>[2x]SMPKPIYSYSILIFMALKN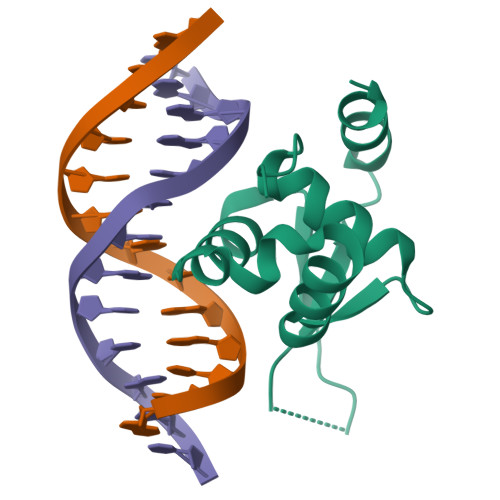SKTGSLPVSEIYNFMTEHFPYFKTAPDGWKNSVRHNLSLNKCFEKVENKSGSSSRKGCLWALNPAKIDKMQEELQKWKRK> MAFYSCCWVLLALTWHTSAYGPDQRAQKKGDIILGGLFPIHFGVAAKDQDLKSRPESVECIRYNFRGFRWLQAMIFAIEEINSSPALLPNLTLGYRIFDTCNTVSKALEATLSFVAQNKIDSLNLDEFCNCSEHIPSTIAVVGATGSGVSTAVANLLGLFYIPQVSYASSSRLLSNKNQFKSFLRTIPNDEHQATAMADIIEYFRWNWVGTIAADDDYGRPGIEKFREEAEER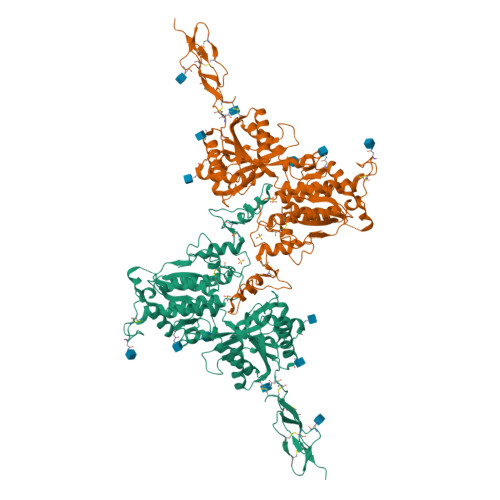DICIDFSELISQYSDEEEIQHVVEVIQNSTAKVIVVFSSGPDLEPLIKEIVRRNITGKIWLASEAWASSSLIAMPQYFHVVGGTIGFALKAGQIPGFREFLKKVHPRKSVHNGFAKEFWEETFNCHLQEGAKGPLPVDTFLRGHEESGDRFSQSSTAFRPLCTGDENINSVETPYIDYTHLRISYNVYLAVYSIAHALQDIYTCLPGRGLFTNGSCADIKKVEAWQVLKHLRHLNFTNNMGEQVTFDECGDLVGNYSIINWHLSPEDGSIVFKEVGYYNVYAKKGERLFINEEKILWSGFSREVPFSNCSRDCLAGTRKGIIEGEPTCCFECVECPDGEYSDETDASACNKCPDDFWSNENHTSCIAKEIEFLSDYKDDDDK> X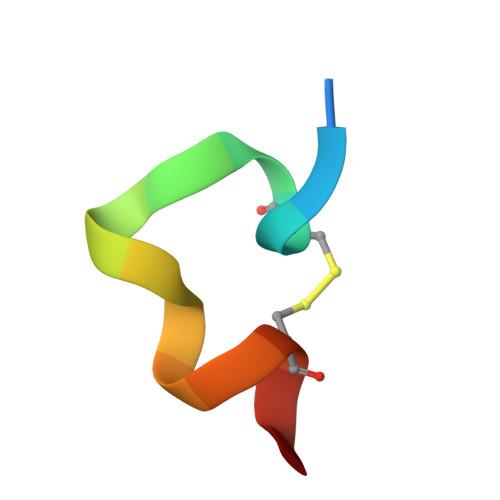KGACDYPEWQWLCAAX N-{[2-(dimethylamino)pyridin-4-yl]methyl}acetamide | C10 H15 N3 O | 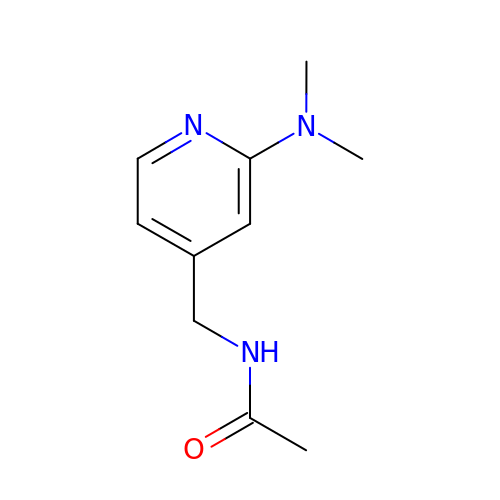BKIVWGJUNJZCKF-UHFFFAOYSA-N>GMSLKSTTSSLTTNNHDKTINSVQSLVNGTGTVADHNPYDEVPYESYPYAITNPYHLSTLATLFGINAPEVENSKILELGCAAGGNLIPHAVLYPNAHFVGVDLSKVQIDEANKNVRALGLKNIEFHHCSITDIDDSFGKFDYIICHGVISWVPKIVRDKIFKVCNRNLSTNGIAYISYNTLPGWNMVRTIRDMMLYHSSSFTNIRDRIAQSRLLLEFVKDSLEHSKTPYAEVLKTEAGLLAKQTDHYLRHDHLEEE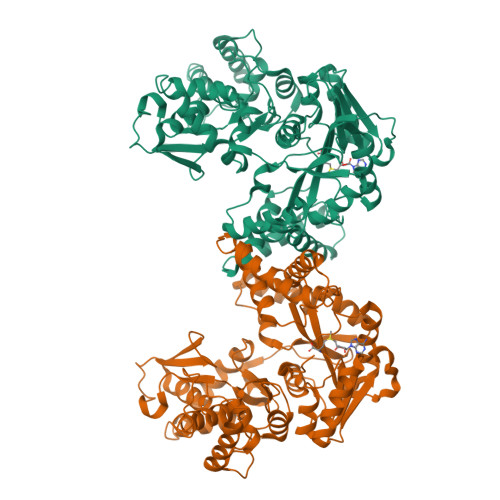NAQFYFHEFMNEARKHNLQYLADCNISTMYLGNMPPKVVEQLKAVNDIVRTEQYMDFITNRRFRTTLLCHNDLKINRNINNDDIKKFNIIFNVIPEKPLKEVDLNNATENLQFFLNGNKESNLSTTSPYMKAILYTFSENLNNPLSFKQVTSEANTKLNNTKLNEIKNELLNNAMKLVLQGYISITNQKHRSKPVLDKPKTTQMVIYQAKYTPSMWVTNLKHEPIGVNFFEKFALRYMDGRNDKKAIIEAILGHVEKGELTLSREGQKIENKEEIRKELESLFTPMIEKFCSNALLV[2x]>SNAMTALKVGSESWWQSKHGPEWQRLNDEMFEVTFWWRDPQGSEEYSTIKRVWVYITGVTDHHQNSQPQSMQRIAGTDVWQWTTQLNANWRGSYCFIPTERDDIFSAPSPDRLELREGWRKLLPQAIADPLNPQSWKGGLGHAVSALEMPQAPLQPGWDCPQAPEIPAKEIIWKSERLKNSRRVWIFTTGDVTAEERPLAVLLDGEFWAQSMPVWPVLTSLTHRQQLPPAVYVLIDAIDTTHRAHELPCNADFWLAVQQELLPLVKVIAPFSDRADRTVVAGQSFGGLS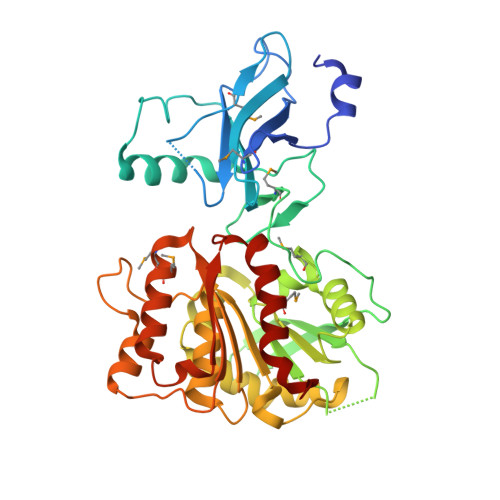ALYAGLHWPERFGCVLSQSGSYWWPHRGGQQEGVLLEKLKAGEVSAEGLRIVLEAGIREPMIMRANQALYAQLHPIKESIFWRQVDGGHDALCWRGGLMQGLIDLWQPLFHDRS[4x]>[8x]MPHLLENSWTFWFDTPAAKSKQAAWGSSMRPIYTFSTVEEFWSIYNNIHHPGKLAVGADFYCFKHKIEPKWEDPICANGGKWTANYPKGKSDTSWLYTLLAMIGEQFDHGDEICGAV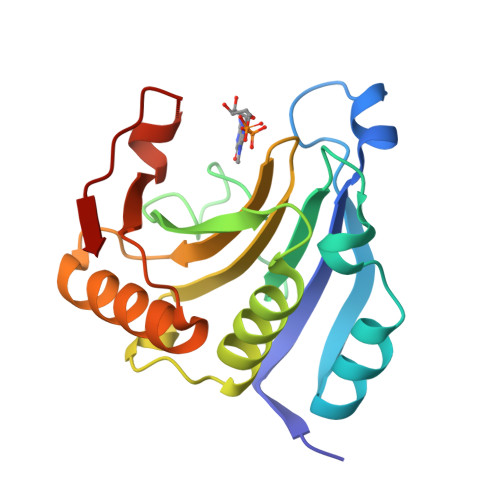VNVRGRAEKISIWTKNASNEAAQVSIGKQWKEFLDYNETMGFIFHDDARKLDRNAKNKYVV Ung (family 1 of the UDG superfamily) is the most prevalent form of UDG and removes uracil bases, regardless of their state of base pairing or sequence context, via the cleavage of the glycosyl bond attaching them to the deoxyribose. Ung inhibitors (which are interchangeably referred to herein as UngIns) are DNA mimetic proteins utilising charge-based alignment with the Ung DNA binding cleft to dock Ung. Docking promotes the hydrophobic sequestration of the sidechain of the apical residue in the Ung DNA minor groove binding loop, which is essentially irreversible under biological conditions, to inhibit Ung. UngIn protein structures described to date fall into one of three observed folds: Ugi/SAUGI (note that Ugi and SAUGI share the same protein fold at ~12% sequence residue identity), p56, and Vpr; yet, within each fold, type there is pronounced sequence plasticity, to the extent that the unambiguous identification of an Ung inhibitor in any genome is rarely straightforward.

Of these, the most distantly related to structurally characterised p56 proteins is a sequence encoded by Bacillus phage VMY22 (“VMY22_4”; Gene ID: 26625151), with a sequence identity of 23% to Bacillus phage PZA p56. The VMY22 open reading frame sequence was synthetically optimised for E. coli and recombinantly expressed. The protein was biochemically validated to act as an UngIn and confirmed as a structural homolog of previously characterised p56 proteins. PZA p56 and VMY22 p56 variants show structural conservation (RMSD = 0.883 Å) despite low sequence identity (24%). The primary difference of note is a deeper inhibitory hydrophobic pocket in the VMY22 p56 variant, due to tryptophan in the 3rd β-strand functionally substituting a helix-located side chain that is a phenylanaline in PZA p56. In VMY22 p56, that phenylalanine is a cysteine and does not form part of the hydrophobic pocket. Other sequence changes do not contribute to significant observed structural differences. Furthermore, crystal structures were determined for each variant in complex with Ung and revealed fold conservation with PZA p56, SAUGI, and Ugi.

>[4x]MENVLKNDWGPLLATEFEKEYYRKLADFLKEEYSTHVVYPKVEDIFNALQYTSYENTKVVILGQDPYHGPNQAHGLSFSVQPGVKTPPSLLNMYKELRDEYGYEIPNNGYLVKWAEQGVLLLNTVLTVRQSEANSHKGKGWEHFTDRVIELLNEREKPVIFILWGRHAQAKKKLITNPNHHIIESVHPSPLSARRGFFGSKPYSKVNTILANMGEREIDWEIPNL;>MEGFKDSYTLIYVTRDEEGKMFDIKLENQTKEECEIIYGMITDEILIWNMILEGMF[8x]>[8x]NSELDRLSKDDRNWVMQTKDYSATHFSRLTEINSHNVKNLKVAWTLSTGTLHGHEGAPLVVDGIMYIHTPFPNNVYAVDLNDTRKMLWQYKPKQNPAARAVACCDVVNRGLAYVPAGEHGPAKIFLNQLDGHIVALNAKTGEEIWKMENSDIAMGSTLTGAPFVVKDKVLVGSAGAELGVRGYVTAYNIKDGKQEWRAYATGPDEDLLLDKDFNKDNPHYGQFGLGLSTWEGDAWKIGGGTNWGWYAYDPKLDMIYYGSGNPAPWNETMRPGDNKWTMTI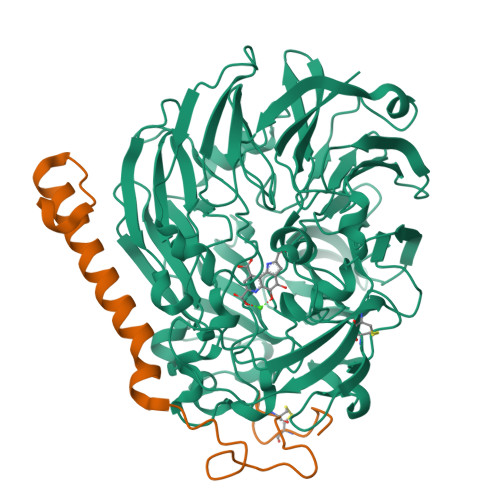WGRDADTGRAKFGYQKTPHDEWDYAGVNYMGLSEQEVDGKLTPLLTHPDRNGLVYTLNRETGALVNAFKIDDTVNWVKKVDLKTGLPIRDPEYSTRMDHNAKGICPSAMGYHNQGIESYDPDKKLFFMGVNHICMDWEPFMLPYRAGQFFVGATLNMYPGPKGMLGQVKAMNAVTGKMEWEVPEKFAVWGGTLATAGDLVFYGTLDGFIKARDTRTGELKWQFQLPSGVIGHPITYQHNGKQYIAIYSGVGGWPGVGLVFDLKDPTAGLGAVGAFRELAHYTQMGGSVFVFSL;>YDGTHCKAPGNCWEPKPGYPDKVAGSKYDPKHDPNELNKQAESIKAMEARNQKRVENYAKTGKFVYKVEDIK[8x]>[2x]MPREYEFAEKILFTEEEIRTRIKEVAKRIADDYKGKGLRPYVNPLVLISVLKGSFMFTADLCRALCDFNVPVRMEFICVSSYGEGLTSSGQVRMLLDTRHSIEGHHVLIVEDIVETALTLN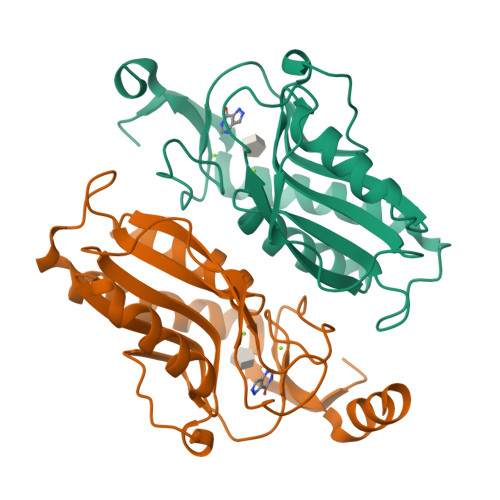YLYHMYFTRRPASLKTVVLLDKREGRRVPFSADYVVANIPNAFVIGYGLDYDDTYRELRDIVVLRPEVYAEREAARGKKQRAIGSADTDRDAKREFHSKY> SGSGSWQSYVDNQICQHVDCRLAVIAGLQDGAVWAKFEKDLPKQITQQELKTIADAIRSNPNSFLEGGIHLGGEKYICIQADNSLVRGRKGSSALCIVATNTCLLAAA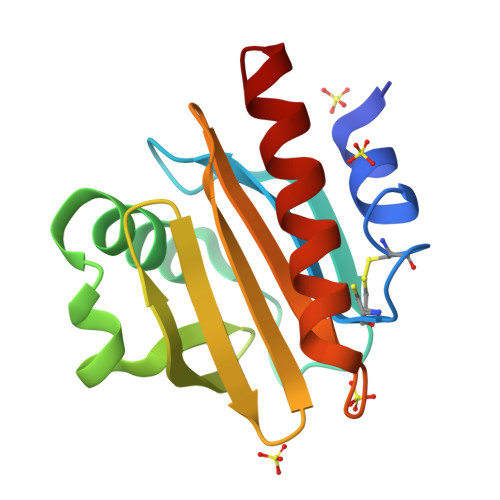TVDGFPPGQLNNVVEKLGDYLKANNY>MKVNRPAERASFGSFVLDAGSARFVGSDELALVLGFAPGDVVLTPAVVLAHLHPDDRLEWQAGLQRCLATGRPVVVNHLL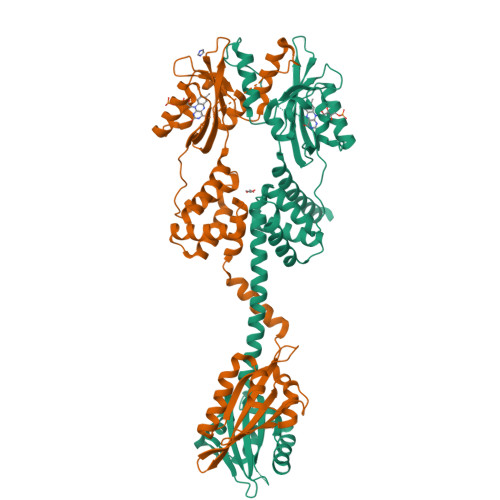LTAEAEPRPAMTTLTALTEQDRVRAVTGVITDLSDRVRRATEAEIRQAVRAAAATRSEIDQAKGIVMAAFDVDADQAFALLKWHSSQSNRKLRDLATGMIEGLAAANSALPLRRRLSTVFTDMGCPAPSTKGWTVPVTDIGLPPTSGLIPTALLPGILTRAAHDASVAITVADVTAPDQPLVYANPAFERLTGYAAAEVLGRNCRFLQAESGDPHERSAIRSAIANGDAVTTLIRNFRQDGHAFWNEFHLSPVRNGAGRVTHYIGYQLDVTERVERDQQLEQLASLEHHHHHH[4x]N-(trifluoroacetyl)-beta-D-glucopyranosylamine | C8 H12 F3 N O6 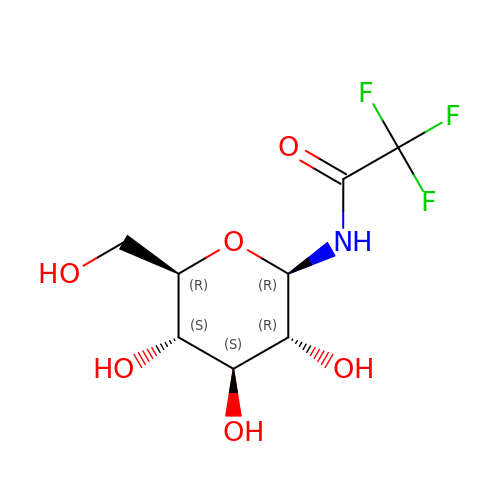| XMUBEPVSEUVEBW-VFUOTHLCSA-N> MTAVQLIV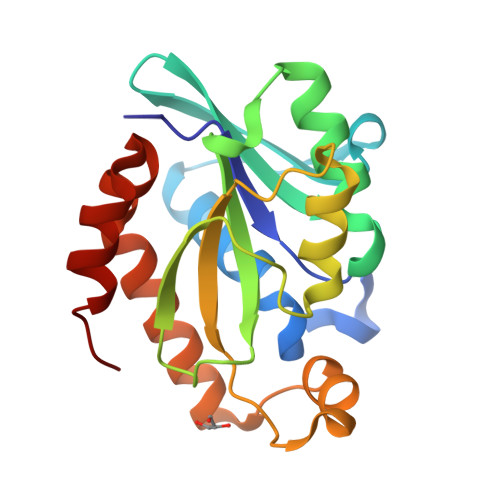GLGNPGPEYDQTRHNAGALFVERLAHAQGVSLVADRKYFGLVGKFSHQGKDVRLLIPTTYMNRSGQSVAALAGFFRIAPDAILVAHDELDMPPGVAKLKTGGGHGGHNGLRDIIAQLGNQNSFHRLRLGIGHPGHSSLVSGYVLGRAPRSEQELLDTSIDFALGVLPEMLAGDWTRAMQKLHSQKA N-[(1R)-1-(4-fluorophenyl)ethyl]-N'-[(2S,3S)-3-hydroxy-1-phenyl-4-(1H-pyrazol-1-yl)butan-2-yl]-5-[methyl(methylsulfonyl)amino]benzene-1,3-dicarboxamide 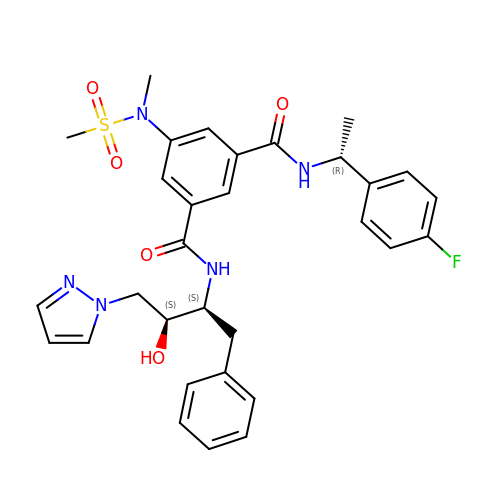| C31 H34 F N5 O5 S | YTBFVFURRJQMRL-AUDJAPFVSA-N>[2x]MAEKPKLHYFNARGRMESTRWLLAAAGVEFEEKFIKSAEDLDKLRNDGYLMFQQVPMVEIDGMKLVQTRAILNYIASKYNLYGKDMKERALIDMYSE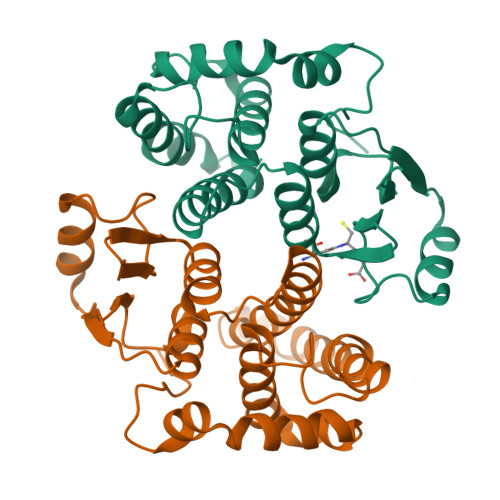GILDLTEMIIQLVICPPDQREAKTALAKDRTKNRYLPAFEKVLKSHGQDYLVGNRLTRVDIHLLELLLYVEEFDASLLTSFPLLKAFKSRISSLPNVKKFLQPGSQRKPAMDAKQIEEARKIFRF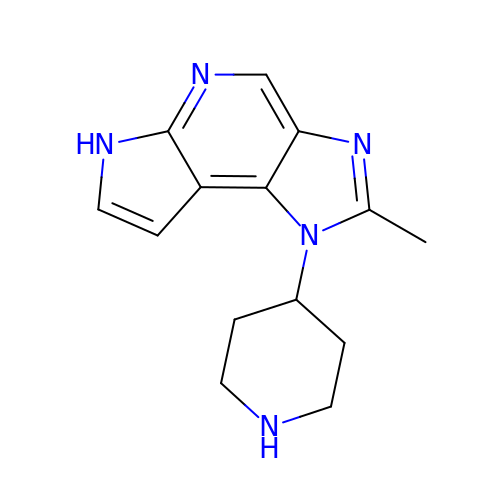2-methyl-1-(piperidin-4-yl)-1,6-dihydroimidazo[4,5-d]pyrrolo[2,3-b]pyridine | C14 H17 N5 | XTQACRIFOIASKV-UHFFFAOYSA-N> MKYLVLVLCLTSCACRDIGLWTFRYVY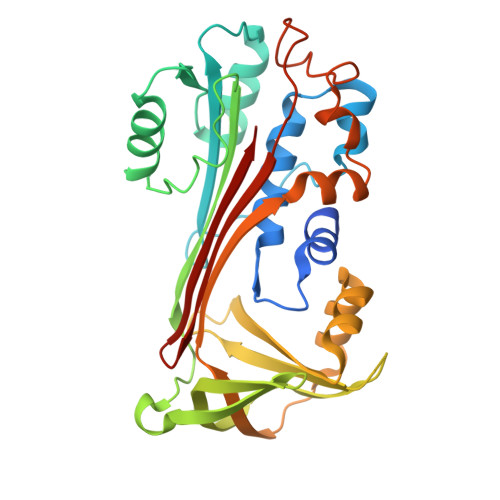NESDNVVFSPYGLTSALSVLRIAAGGNTKREIDVPESVVEDSDAFLALRELFVDASVPLRPEFTAEFSSRFNTSVQRVTFNSENVKDVINSYVKDKTGGDVPRVLDASLDRDTKMLLLSSVRMKTSWRHVFDPSFTTDQPFYSGNVTYKVRMMNKIDTLKTETFTLRNVGYSVTELPYKRRQTAMLLVVPDDLGEIVRALDLSLVRFWIRNMRKDVCQVVMPKFSVESVLDLRDALQRLGVRDAFDPSRADFGQASPSNDLYVTKVLQTSKIEADERGTTASSDTAIT> TTSSDQKCIEKEVNKTYNCENLGLNEIPGTLPNSTECLEFSFNVLPTIQNTTFSRLINLTFLDLTRCQIYWIHEDTFQSQHRLDTLVLTANPLIFMAETALSGPKALKHLFFIQTGISSIDFIPLHNQKTLESLYLGSNHISSIKLPKGFPTEKLKVLDFQNNAIHYLSKEDMSSLQQATNLSLNLNGNDIAGIEPGAFDSAVFQSLNFGGTQNLLVIFKGLKNSTIQSLWLGTFEDMDDEDISPAVFEGLCEMSVESINLQKHYFFNISSNTFHCFSGLQELDLTATHLSELPSGLVGLSTLKKLVLSANKFENLCQISASNFPSLTHLSIKGNTKRLELGTGCLENLENLRELDLSHDDIETSDCCNLQLRNLSHLQSLNLSYNEPLSLKTEAFKECPQLELLDLAFTRLKVKDAQSPFQNLHLLKVLNLSHSLLDISSEQLFDGLPALQHLNLQGNHFPKGNIQKTNSLQTLGRLEILVLSFCDLSSIDQHAFTSLKMMNHVDLSHNRLTSSSIEALSHLKGIYLNLASNHISIILPS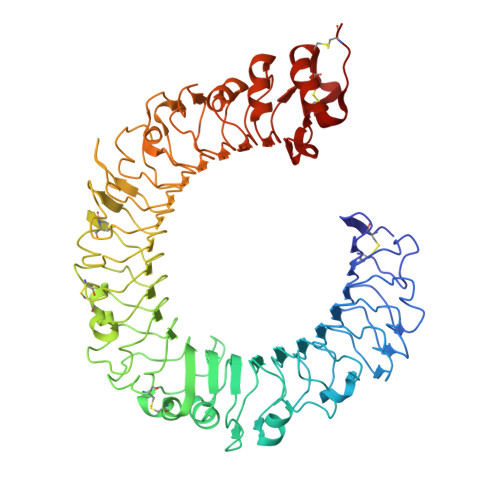LLPILSQQRTINLRQNPLDCTCSNIYFLEWYKENMQKLEDTEDTLCENPPLLRGVRLSDVTLSCS>[2x]MNDAAEVALYERLLQLRVLPGASDVHDVRFVFGDDSRCWIEVAMHGDHVIGNSHPALDPKSRATLEHVLTVQGDLAAFLVVARDML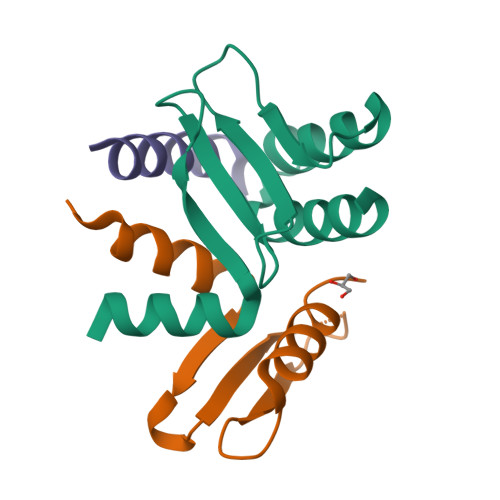LASL;>MANENILKLKLYRSLGVILDLENDQVLINRKNDGNIDILPLDNNLSDFYKTKYIWERLGKHHHHHH[2x];>NKDPNEVRSFLQDLSQVLARKSQGN[2x]> ILEAAVTQSPRNKVAVTGEKVTLS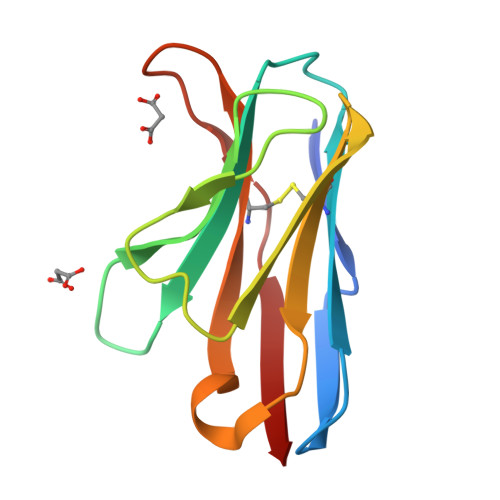CQQTNNHNNMYWYRQDTGHGLRLIHYSYGVGNTEKGDIPDGYEASRPSHEQFSLILVSATPSQSSVYFCASGVGGTLYFGAGTRLSVL> MDVASSDTVYTFPDEFKLGAATASYQIEGAWDENGKGPNIWDTLTHEHPDYVVDGATGDIADDSYHLYKEDVKILKELGAQVYRFSISWARVLPEGHDNIVNQDGIDYYNNLINELLANGIEPMVTMYHWDLPQALQDLGGWPNLV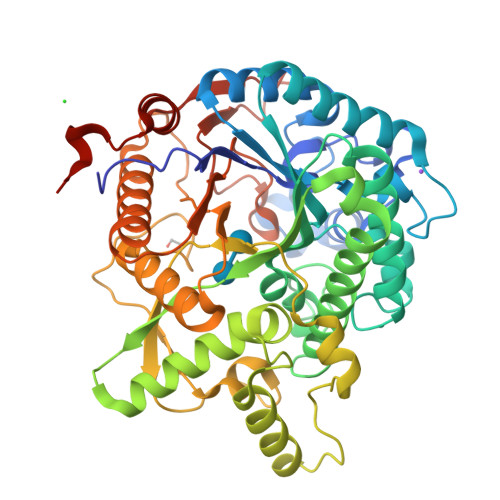LAKYSENYARVLFKNFGDRVKLWLTFNSPLTFMDGYASEIGMAPSINTPGIGDYLAAHTVIHAHARIYHLYDQEFRAEQGGKVGISLNINWCEPATNSAEDRASCENYQQFNLGLYAHPIFTEEGDYPAVLKDRVSRNSADEGYTDSRLPQFTAEEVEYIRGTHDFLGINFYTALLGKSGVEGYEPSRYRDSGVILTQDAAWPISASSWLKVVPWGFRKELNWIKNEYNNPPVFITENGFSDYGGLNDTGRVHYYTEHLKEMLKAIHEDGVNVIGYTAWSLMDNFEWLRGYSEKFGIYAVDFEDPARPRIPKESAKVLAEIMNTRKIPERFRDLEHHHHHH> HHAADYVLYKDATKPVEDRVADLLGRMTLAEKIGQMTQIERLVATPDVLRDNFIGSLLSGGGSVPRKGATAKEWQDMVDGFQKACMSTRLGIPMIYGIDAVHGQNNVYGATIFPHNVGLGATRDPYLVKRIGEATALEVRATGIQYAFAPCIAVCRDPRWGRCYESYSEDRRIVQSMTELIPGLQGDVPKDFTSGMPFVAGKNKVAACAKHFVGDGGTVDGINENNTIINREGLMNIHMPAYKNAMDKGVSTVMISYSSWNGVKMHANQDLVTGYLKDTLKFKGFVISDWEGIDRITTPAGSDYSYSVKASIL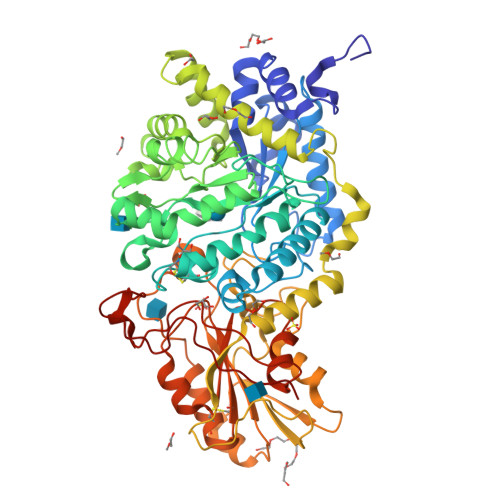AGLDMIMVPNKYQQFISILTGHVNGGVIPMSRIDDAVTRILRVKFTMGLFENPYADPAMAEQLGKQEHRDLAREAARKSLVLLKNGKTSTDAPLLPLPKKAPKILVAGSHADNLGYQCGGWTIEWQGDTGRTTVGTTILEAVKAAVDPSTVVVFAENPDAEFVKSGGFSYAIVAVGEHPYTETKGDNLNLTIPEPGLSTVQAVCGGVRCATVLISGRPVVVQPLLAASDALVAAWLPGSEGQGVTDALFGDFGFTGRLPRTWFKSVDQLPMNVGDAHYDPLFRLGYGLTTNATKKY(6-bromo-2-phenyl-1-benzofuran-3-yl)acetic acid | C16 H11 Br O3 | 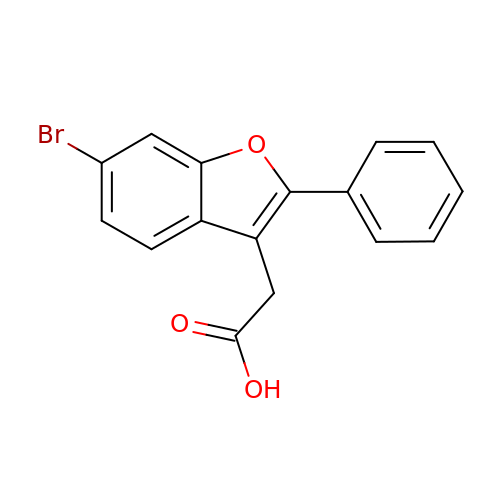GRIUNLJADADECO-UHFFFAOYSA-N6-HYDROXY-7,8-DIHYDRO PURINE NUCLEOSIDE | C10 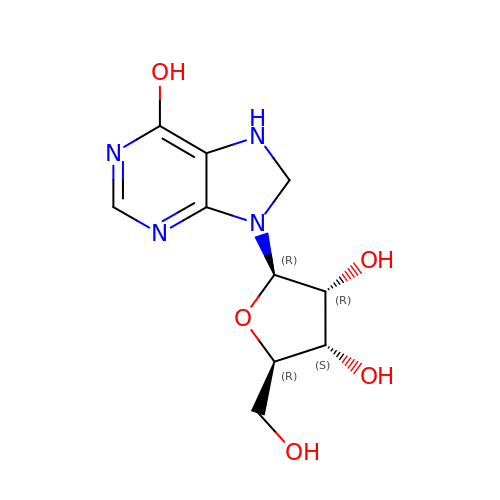H14 N4 O5 | ZWTNXGIZBOQCAJ-KQYNXXCUSA-N>MPLFNSILDTIGRTPIVRLQRMAPEHTSVYVKVESFNPGGSVKDRLALSVVLDAEAKGLLKPGDTIVECTSGNVGIALAMVAAARGYRFVAVMGDTYSVERRKLIRAYGGKLVLFPGHLGSKGG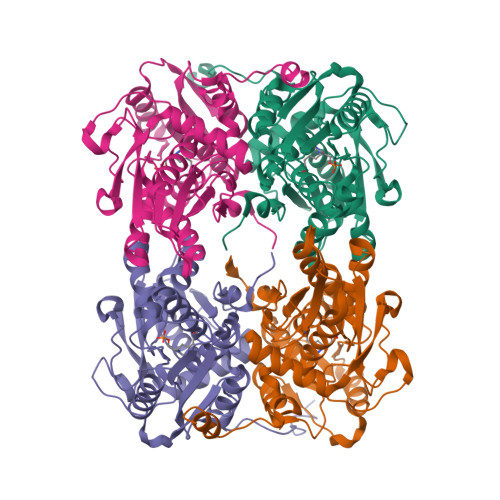NLIADELAEKYGWFRARQFDNPANPSYHRETTASEILADFAGKRLDHFVTGFGTTGTLTGVGQMLRVARPEVRVVALEPSNAAMLARGEWSPHQIQGLAPNFVPGVLDRSVIDDLVTMDEVTARDTSRRLAAEEGIFAGISAGATVATALSIAEHAPEGTVLLAMLPDTGERYLSTFLFDGVDEGSDDAWLASLDTGSGLLEHHHHHH[8x]>[2x]MGHHHHHHSSGRENLYFQGHPVLEKLKAINNYNPKDFDWNLKNGRVFIIKSYSEDDIHRSIKYSIWCSTEHGNKRLDAAYRSLNGKGPLYLLFSVNGSGHFCGVAEMKSVVD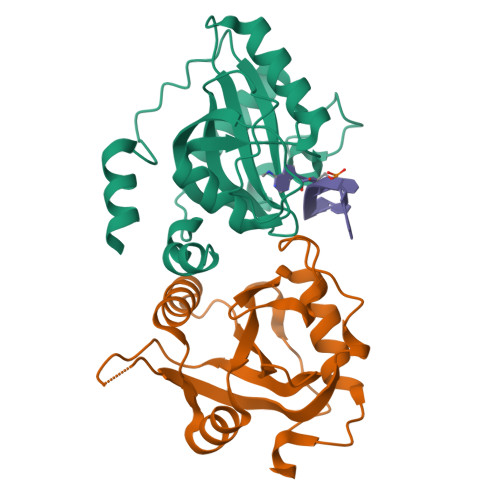YNAYAGVWSQDKWKGKFEVKWIFVKDVPNNQLRHIRLENNDNKPVTNSRDTQEVPLEKAKQVLKIIATFKHTTSIFDDFAHYEKRQE> MTIEKNLSDVQQKYADQFQEDVVKSFQTGYGITPDTQIDAGALRREILDDQITMLTWTNEDLIFYRDISRRPAQSTVVKYDQYLRHGNVG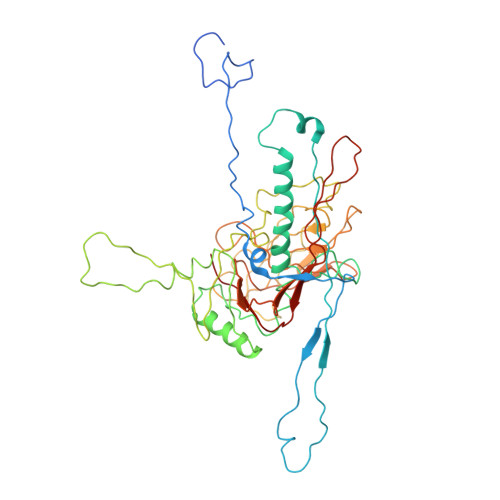HSRFVKEIGVAPVSDPNIRQKTVSMKYVSDTKNMSIASGLVNNIADPSQILTEDAIAVVAKTIEWASFYGDASLTSEVEGEGLEFDGLAKLIDKNNVINAKGNQLTEKHLNEAAVRIGKGFGTATDAYMPIGVHADFVNSILGRQMQLMQDNSGNVNTGYSVNGFYSSRGFIKLHGSTVMENELILDESLQPLPNAPQPAKVTATVETKQKGAFENEEDRAGLSYKVVVNSDDAQSAPSEEVTATVSNVDDGVKLSINVNAMYQQQPQFVSIYRQGKETGMYFLIKRVPVKDAQEDGTIVFVDKNETLPETADVFVGEMSPQVVHLFELLPMMKLPLAQINASITFAVLWYGALALRAPKKWARIKNVRYIAV> SNAMAVLLSGVPVLAALDVSTTQXFWIEVLGFTEEFLTEDFGGVSRDGVELFICSVEDQVVPDNTQAWLRVRDIDALHAEWSARVSSDYADASH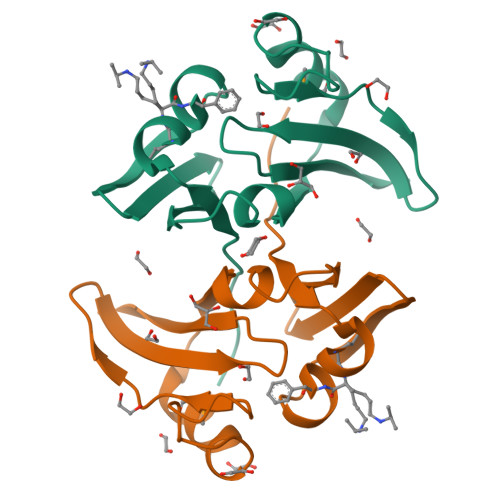PAMTAIREVPWGREFGLRDPAGNLVHFSELSEAAETTRTVR> QVQSVEVMRDSYGVPHVFADSHYGLYYGYGYAVAQDRLFQMDMARRSFVGTTAAVLGPGEQDAYVKYDMQVRQNFTPASIQRQIAALSKDERDIFRGYADGYNAYLEQVRRRPELLPKEYVDFDFQPEPLTDFDVVMIWVGSMANR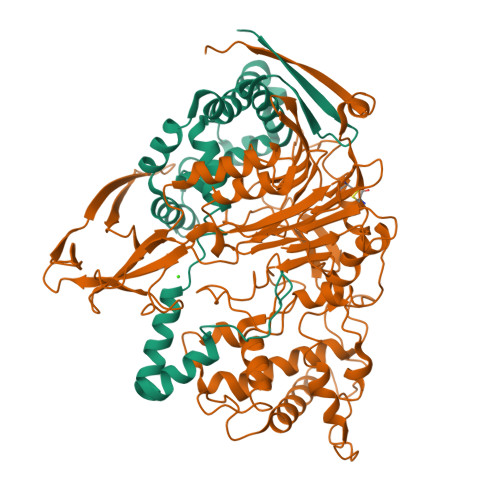FSDTNLEVTALAMRQSLEKQHGPERGRALFDELLWINDTTAPTTVPAPA;> SNLWSTRPERVQEGSTVLINGPQFGWYNPAYTYGIGLHGAGFDVVGNTPFAYPIVLFGTNSEIAWGATAGPQDVVDIYQEKLNPSRADQYWFNNAWRTMEQRKERIQVRGQADREMTIWRTVHGPVMQFDYDQGAAYSKKRSWDGYEVQSLLAWLNVAKARNWTEFLDQASKMAISINWYYADKHGNIGYVSPAFLPQRPADQDIRVPAKGDGSMEWLGIKSFDAIPKAYNPPQGYLVNWNNKPAPDKTNTDTYYWTYGDRMNELVSQYQQKDLFSVQEIWEFNQKASYSDVNWRYFRPHLEKLAQQLPADDSSKAALTMLLAWDGMEQDQGGQNAGPARVLFKTWLEEMYKQVLMPVVPESHRAMYSQTGFATQQGPNPGSINLSMGTKVLLRALVLEAHPDPKRVNVFGERSSQEIMHTALQNAQARLSQEQGAQMARWTMPTSVHRFSDKNFTGTPQTMPGNTFAFTGYQNRGTENNRVVFDAKGVEFCDAMPPGQSGFTDRNGVRSPHYEDQLKLYENFECKTMDVTHADIRRNAQSSTMLLIQPQP> MGKAKK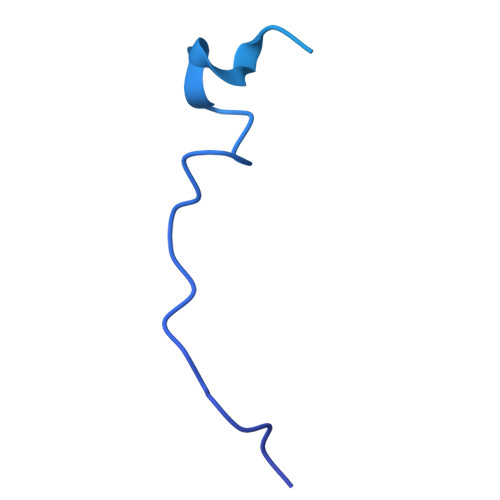TRKFGLVKRTLNTKKDQRLKKNQENIKTKEDPELTRNIPQVSSALFFQYNQAIKPPYQVLIDTNFINFSIQKKVDIVRGMMDCLLAKCNPLITDCVMAELEKLGPKYRIALKLARDPRIKRLSCSHKGTYADDCLVHRVLQHKCYIVATNDAGLKQRIRKIPGIPLMSVGGHAYVIEKLPDVF> SLLNVPAGKDLPEDIYVVIEIPANADPIKYEIDKESGALFVDQFMSTAMFYPCNYGYINHTLSLDGDPVDVLVPTPYPLQPGSVTRCRPVGVLKMTDEAGEDAKLVAVPHSKLSKEYDHIKDVNDLPELLKAQIAHFFEH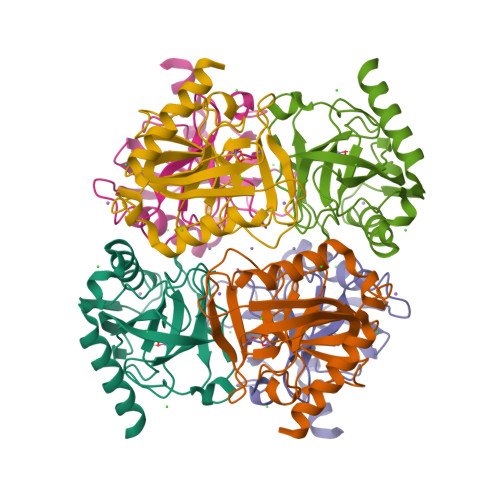YKDLEKGKWVKVEGWENAEAAKAEIVASFERAKNK The replication of RNA viruses relies on the activity of RNA-dependent RNA polymerases (RdRps). Despite large variations in their genomic sequences, viral RdRps share a common architecture generally known as a closed right hand. In most dsRNA viruses, RdRps perform both genome replication and transcription without the need for primers; during replication RdRps use positive-sense single-stranded RNA - (+)ssRNA - transcripts to produced dsRNA, whereas during transcription the produced negative-sense RNA - (-)ssRNA - serves as a template to produce (+)ssRNA copies from the dsRNA template. Although cystoviral P2 RdRps catalyse the same reactions, they have distinct template specificities.

The full-length φ8 P2 structure (residues 2-636) was determined at 3Å resolution by molecular replacement using an AF2 generated search model. The overall structure of φ8 P2 is roughly globular, consisting of 24 α-helices and 19 β-strands. It has a typical RNA polymerase fold and resembles a cupped right hand with finger, thumb and palm subdomains, which together form the active site of the enzyme. Despite the low sequence identity, the overall fold of φ8 P2 is similar to that of φ6 P2 (Root mean square deviation (RMSD) of the Cα atoms over 540 residues: 2.1Å) and φ12 P2 (RMSD of the Cα atoms over 534 residues: 2.1Å) and displays all the conserved structural features of RdRps. The main difference between φ8 P2 and the other two P2 structures appears to be in the first 50 residues at the N-terminus. Within the thumb subdomain, a notable variation is observed where a compact loop consisting of four residues in φ6 and φ12 P2, is substituted with an elongated β-hairpin structure spanning eleven residues (β2-β3) in φ8 P2. Because of the high concentration of CaCl2 in the crystallisation condition, a Ca2+ ion was modelled at the non-catalytic ion site of the φ8 P2 structure. The Ca2+ ion is coordinated by the sidechains of three aspartate residues (D323, D446, D475) as well as the main-chain carbonyl of lysine K479. In φ8 P2, the presence of Ca2+ ions could lock D323 into an inactive conformation, coordinating the non-catalytic site instead of the catalytic site, that hinders its ability to catalyse the reaction.

> MASFVPLVGDPKLEGSYFSWVNNQPSAMDDYSLVKTVAAIRTAFGPSINRAPSFKDVTQLVVVTRTGVKHYKANDPQYLRFQKELADALQQFEPSKQLTLGVTGLGLTRDFGTMYTHGAVFMNPTLSPRVDRLGETGGELPSDYMLALSIMSEIYFEEFKPAKVRTNGKSKTGLPNNTKDAREKKKFFMSLMDHGTGWSSALAKGDYSYSAKYYGSAPITLPTYRDQLEKPGKKRDGYDFLGNAVVAADKSIPSKYSQGVDGLHALRRRTAYAVSYAAATPMQCFVAGCRHIALERYGETWHEHDAEDIIRRIYKYGFYELYDASAFDTGFSWKEITTMIDAIPGITDLARDYMRSVHRLPLLITSDVRGVKGAYLLNMDKYSPGLQSGVPSVSDFGKIRGAAQWSYGLMVLGAIRYQSRAQLKTEFKTLLKHGRPDFAMQNRGDDTMPLAARQKDLQKWCEIVEGFKFCKWEKDTGKKFIGRVLYQRTPESKVVAYSDIVTMLEKTFINERSMFSAHRPFAATGNVMRYEMNMAHPAFGAVMDVVDTIMLKHFGVTYKECFVGAQALEKELNNGVELPDYAGLNQATRDFILDPDVIHYKWRESDIDPRVLDMVMPTSLEPDLCEEAVHKFGFVK> LTIGNSTITTQEAANIIVGYGEWPSYCSDTRPDVSVNRFYTLDTKLWEKSSKGWYWKFPDVLTETGVFGQNAQFHYLYRSGFCIHVQCNASKFHQGALLVAVLPEYVIGTVAGGTGTEDSHPPYKQTQPGADGFELQHPYVLDAGIPISQLTVCPHQWINLRTNNCAT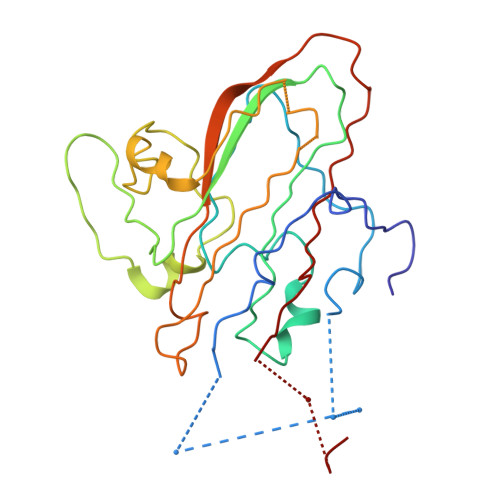IIVPYINALPFDSALNHCNFGLLVVPISPLDYDQGATPVIPITITLAPMCSEFAGLRQ>[2x]GSGIFPKVATNIMRAWLFQHLTHPYPSEEQKKQLAQDTGLTILQVNNWFINA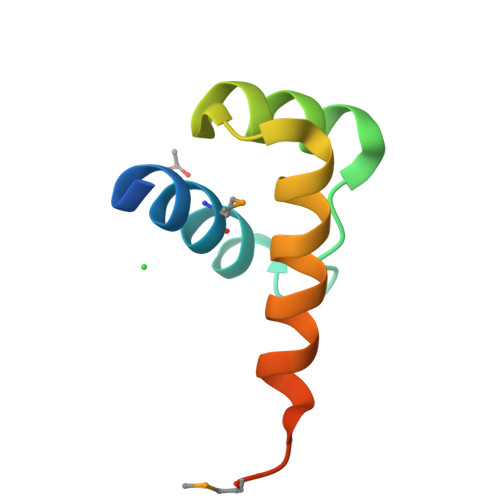RRRIVQPMIDQSNRA> AVKLAPPTDVRSGYIRLVKNVNYYIDSESIWVDNQEPQI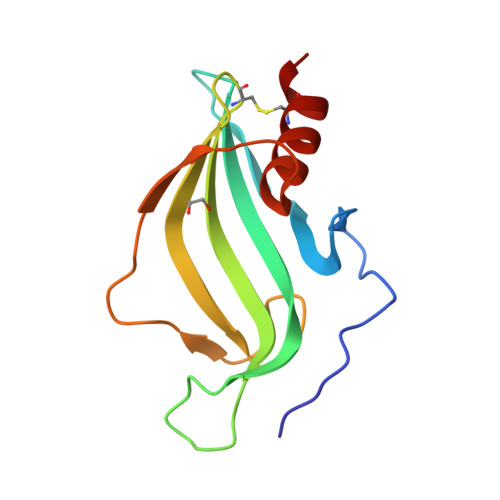VHFDAVVNLDKGLYVYPEPKRYARSVRQYKILNCANYHLTQVRTDFYDEFWGQGLRAAPKKQKKHTLSLTPDTTLYNAAQIICANYGK;> AAVKLAPPTDVRSGYIRLVKNVNYYIDSESIWVDNQEPQIVHFDAVVNLDKGLYVYPEPKRYARSVRQYKILNCANYHLTQVRTDFYDEFWGQGLRAAPKKQKKHTLSLTPDTTLYNAAQIICANYGEA> MVKLAEFSRTATFAWSHDKIPLLVSGTVSGTVDANFSTDSSLELWSLLAADSEKPIASLQVDSKFNDLDWSHNNKIIAGALDNGSLELYSTNEANNAINSMARFSNHSSSVKTVKFNAKQDNVLASGGNNGEIFIWDMNKCTESPSNYTPLTPGQSMSSVDEVISLAWNQSLAHVFASAGSSNFASIWDLKAKKEVIHLSYTSPNSGIKQQLSVVEWHPKNSTRVATATGSDNDPSILIWDLRNANTPLQTLNQGHQKGILSLDWCHQDEHLLLSSGRDNTVLLWNPESAEQLSQFPARGNWCFKTKFAPEAPDLFACASFDNKIEVQTLQNLTNTLDEQETETKQQESETDFWNNVSREESKEKPTVFHLQAPTWYGEPSPAAHWAFGGKLVQITPDGKGVSITNPKISGLESNTTLSEALKTKDFKPLINQRLVKVIDDVNEEDWNLLEKLSMDGTEEFLKEALAFDNDESDAQDDANNEKEDDGEEFFQQIETNFQPEGDFSLSGNIEQTISKNLVSGNIKSAVKNSLENDLLMEAMVIALDSNNERLKESVKNAYFAKYGSKSSLSRILYSISKREVDDLVENLDVSQWKFISKAIQNLYPNDIAQRNEMLIKLGDRLKENGHRQDSLTLYLAAGSLDKVASIWLSEFPDLEDKLKKDNKTIYEAHSECLTEFIERFTVFSNFINGSSTINNEQLIAKFLEFINLTTSTGNFELATEFLNSLPSDNEEVKTEKARVLIASGKSLPAQNPATATTSKAKYTNAKTNKNVPVLPTPGMPSTTSIPSMQAPFYGMTPGASANALPPKPYVPATTTSAPVHTEGKYAPPSQPSMASPFVNKTNSSTRLNSFAPPPNPYATATVPATNVSTTSIPQNTFAPIQPGMPIMGDYNAQSSSIPSQPPINAVSGQTPHLNRKANDGWNDLPLKVKEKPSRAKAVSVAPPNILSTPTPLNGIPANAASTMPPPPLSRAPSSVSMVSPPPLHKNSRVPSLVATSESPRASISNPYAPPQSSQQFPIGTISTANQTSNTAQVASSNPYAPPPQQRVATPLSGGVPPAPLPKASNPYAPTATTQPNGSSYPPTGPYTNNHTMTSPPPVFNKPPTGPPPISMKKRSNKLASIEQNPSQGATYPPTLSSSASPLQPSQPPTLASQVNTSAENVSHEIPADQQPIVDF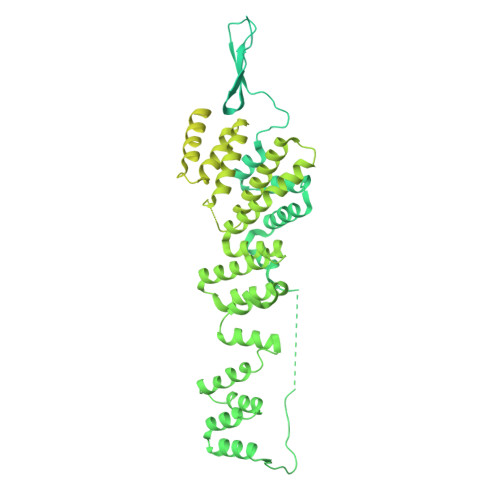LKEELARVTPLTPKEYSKQLKDCDKRLKILFYHLEKQDLLTQPTIDCLHDLVALMKEKKYKEAMVIHANIATNHAQEGGNWLTGVKRLIGIAEATLN> MRLARTLHHVASATTGGGQMLEGLVNDGPEVAHKQHASFTPFSIQPWQARCVGASRRKLLPQMLMYHGARLGPRPLIILDHSTKGEAGVAEAARKYESILSQLSWDYGAVY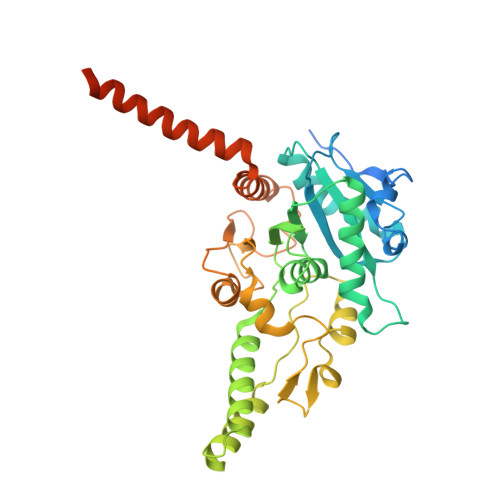IPLHAQCTDSSKDLLEQSCQRICAVMDALDVRWTHFLTYSYGALVAVRMASSQEFPHRVGTLMSLDTPLVTREFLRNMEQREDIAKAERDINVPEDGLAFAKQALLSSLEGPLPCPAAEDESLYRDYLFDPNRIFGAGGLVRDESRYVPLKSLLGVRHPVQLIVPSANPLSDAAAHSEVFGHRRPAVVKCCQRHEDLFKESAAKEVAGVLGAWMRRFEPDCFISKRYEQAANEMGQLMLSTAQVSSESAGKGGGEPRKKKEKKKSKA>[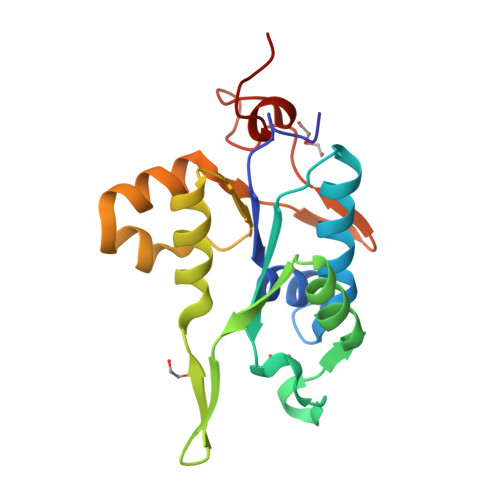2x]DDGENLRPVVIDGSNVAMSHGNKEVFSCRGIKLAVDWFLERGHKDITVFVPAWRKEQSRPDALITDQEILRKLEKEKILVFTPSRRVQGRRVVCYDDRFIVKLAFESDGIIVSNDNYRDLANEKPEWKKFIDERLLMYSFVNDKFMPPDDPLGRHGPSLDNFLRKKPIV Secretory (S) Immunoglobin (Ig) A is the predominant, mammalian mucosal antibody; it is a polymeric antibody assembled in plasma cells that link two IgA monomers and a single copy of the joining chain (JC) to form dimeric (d) IgA (and to a lesser extent, higher order polymers). The pIgR uses five Ig-like domains (D1-D5) and a cytoplasmic tail to bind and transcytose JC-containing antibodies to the apical surface of epithelial cells; there, the pIgR ectodomain, called secretory component (SC), is proteolytically cleaved, releasing the SC-dIgA complex into the mucosa where it is called SIgA (Stadtmueller et al., 2016a). The IgA CH3 contains a C-terminal extension called the tailpiece (Tp), which along with the JC, is required for IgA dimerization and subsequent pIgR binding. Our work describes the structures of mouse SIgA and its precursor, dIgA, which lacks the SC.

To investigate SC’s contribution to the conformation of SIgA, we determined a 3.3 Å average resolution cryoEM structure of dIgA, which contained the same components as SIgA, except for SC. The dIgA structure revealed two IgA monomers arranged similar to those in SIgA; Fabs were disordered. The centroid axes of FcAB and FcCD were bent 98 degrees relative to each other (compared to 97 degrees in SIgA), and the centroid planes were tilted at an angle of 19 degrees (compared to 30 degrees in SIgA). These results suggest that the bend in SIgA is conferred by JC binding to heavy chains and/or interactions between the Tps from both antibodies. The 11-degree difference in tilt between the two structures suggests that SC binding can influence the conformational relationship between the two IgAs. Aligned individually, the structures of the heavy chains and JC were largely superimposable with equivalent chains in SIgA; however, differences were apparent in regions that are bound by SC in SIgA. In particular, TpD, which forms part of the SC D1-JC interface in SIgA, adopts a different conformation, and the three C-terminal residues are disordered. The three C-terminal residues of JC (Tyr-Pro-Asp), which bind SC D1 CDR1 in SIgA, are also disordered in dIgA. While SC may play a role in stabilizing the conformation of SIgA, the dIgA structure suggests that SC binding induces relatively small changes in the bent and tilted relationship between the two IgAs. In the SIgA and dIgA structures, two of the four accessible sites are occluded by JC wing interactions with CH3A and CH3C.

>WGQGTLVTVSAESARNPTIYPLTLPPALSSDPVIIGCLIHDYFPSGTMNVTWGKSGKDITTVNFPPALASGGRYTMSSQLTLPAVECPEGESVKCSVQHDSNPVQELDVNCSGPTPPPPITIPSCQPSLSLQRPALEDLLLGSDASITCTLNGLRNPEGAVFTWEPSTGKDAVQKKAVQNSCGCYSVSSVLPGCAERWNSGASFKCTVTHPESGTLTGTIAKVTVNTFPPQVHLLPPPSEELALNELLSLTCLVRAFNPKEVLVRWLHGNEELSPESYLVFEPLKEPGEGATTYLVTSVLRVSAETWKQGDQYSCMVGHEALPMNFTQKTIDRLSGKPTNVSVSVIMSEGDGICY[4x];> DDEATILADNKCMCTRVTSRIIPSTEDPNEDIVERNIRIVVPLNNRENISDPTSPLRRNFVYHLSDVCKKCDPVEVELEDQVVTATQSNICNEDDGVPETCYMYDRNKCYTTMVPLRYHGETKMVQAALTPDSCYPD>[2x]GPGDQRFGDLVFRQLAPNVWQHTSYLDMPGFGAVASNGLIVRDGGRVLLVDTAWTDDQTAQILNWIKQEINLPVALAVVTHAHQDKMGGMDALH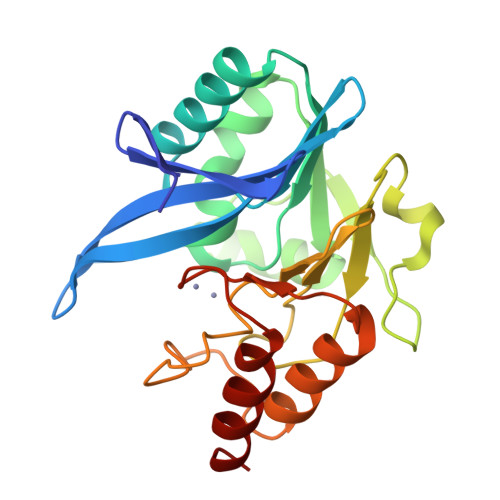AAGIATYANALSNQLAPQEGLVAAQHSLTFAANGWVEPATAPNFGPLKVFYPGPGHTSDNITVGIDGTDIAFGGCLIKDSKAKSLGNLGDADTEHYAASARAFGAAFPKASMIVMSHSAPDSRAAITHTARMADKLR> VEATAQETDRPRFSFSIAAREGKARTGTIEMKRGVIRTPAFMPVGTAATVKALKPETVRATGADIILGNTYHLMLRPGAERIAKLGGLHSFMGWDRPILTDSGGFQVMSLSSLTKQSEEGVTFKSHLDGSRHMLSPERSIEIQHLLGSDIVMAFDEVTPYPATPSRAASSMERSMRWAKRSRDAFDSRKEQAENAALFGIQQGSVFENLRQQSADALAEIGFDGYAVGGLAGGEGQDEMFRVLDFSVPMLPDDKPHYLMGVGKPDDIVGAVERGIDMFDCVLPTRSGRNGQAFTWDGPINIRNARFSED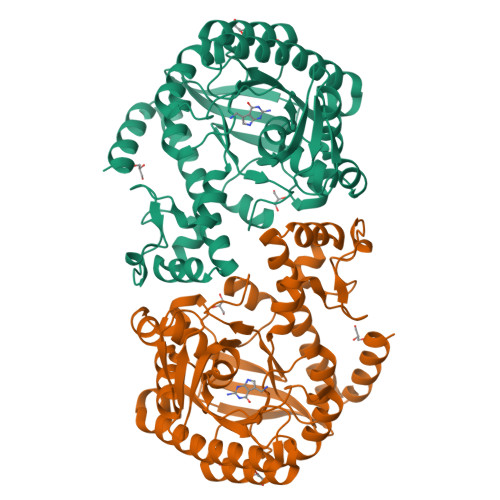LKPLDSECHCAVCQKWSRAYIHHLIRAGEILGAMLMTEHNIAFYQQLMQKIRDSISEGRFSQFAQDFRARYFARNS2-ISOBUTYL-3-METHOXYPYRAZINE | C9 H14 N2 O 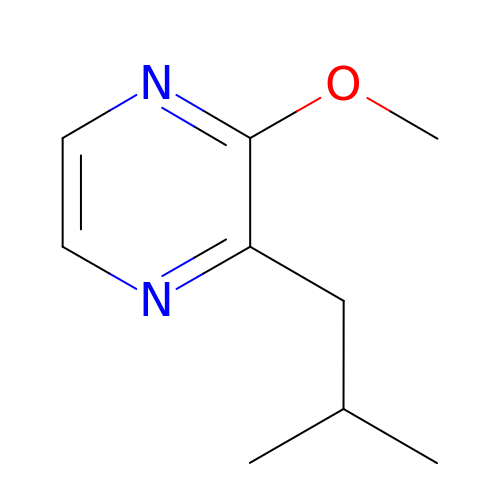| UXFSPRAGHGMRSQ-UHFFFAOYSA-N>MAETKIVVGPQPFSVGEEYPWLAERDE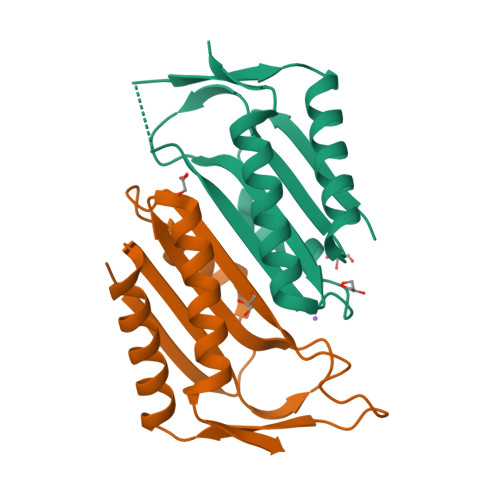DGAVVTFTGKVRNHNLGDSVNALTLEHYPGMTEKALAEIVDEARNRWPLGRVTVIHRIGELWPGDEIVFVGVTSAHRSSAFEAGQFIMDYLKTRAPFWKREATPEGDRWVEAR[6x]>MDIKELHVKTVKRGENVTMECSMSKVKDKNKLAWYRQSFGKVPQYFVRYYSSNSGYKFAEGFKDSRFSMTVNDQKFDLNIIGTREDDGGEYFCGEVEGNTI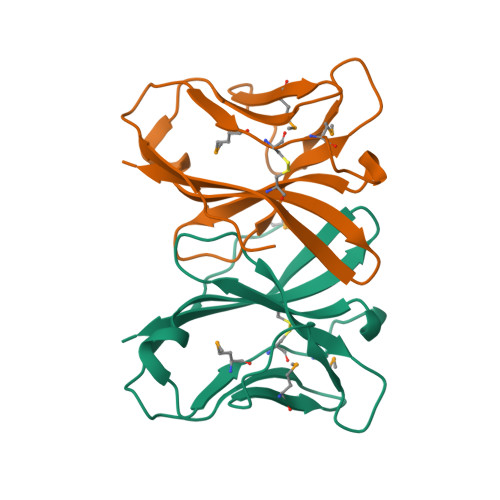KFTSGTRLQF[5x]> KPAKPAAKSIVTLDVKPW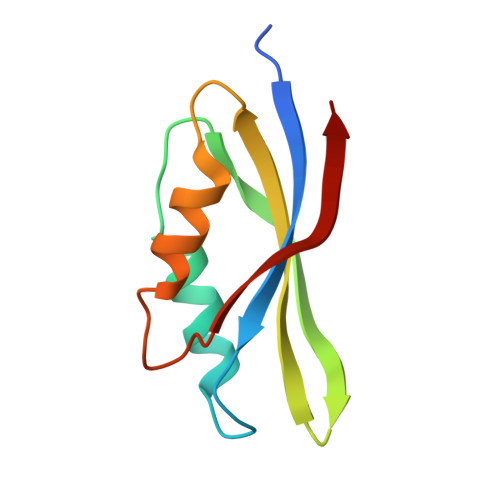DDETNLEEMVANVKAIEMEGLTWGAHQFIPIGFGIKKLQINCVVEDDKVSLDDLQQSIEEDEDHVQSTDIAAMQAL>AECSVD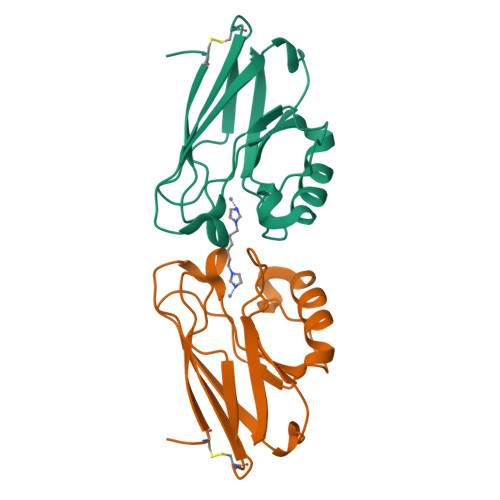IQGNDQMQFNTNAITVDKSCKQFTVNLSHPGNLPKNVMGHNWVLSTAADMQGVVTDGMASGLDKDYLKPDDSRVIAHTKLIGSGEKDSVTFDVSKLKEGEQYMFFCTFPGGSALMKGTLTLK[4x]>MAKKTLPAGVKSPPYIFSPIPFLGHAIAFGKSPIEFLENAYEKYGPVFSFTMVGKTFTYLLGSDAAALLFNSKNEDLNAEDVYSRLTTPVFGKGVAYDVPNPVFLEQKKMLKSGLNIAHFKQHVSIIEKETKEYFESWGESGEKNVFEALSELIILTASHCLHGKEIRSQLNEKVAQLYADLDGGFSHAAWLLPGWLPLPSFRRRDRAHREIKDIFYKAIQKRRQSQEKIDDILQTLLDATYKDGRPLTDDEVAGMLIGLLLAGQHTSSTTSAWMGFFLARDKTLQKKCYLEQKTVCGENLPPLTYDQLKDLNLLDRCIKETLRLRPPIMIMMRMARTPQTVAGYTIPPGHQVCVSPTVNQRLKDSWVERLDFNPDRYLQDNPASGEKFAYVPFGAGRHRCIGENFAYVQIKTIWSTMLRLY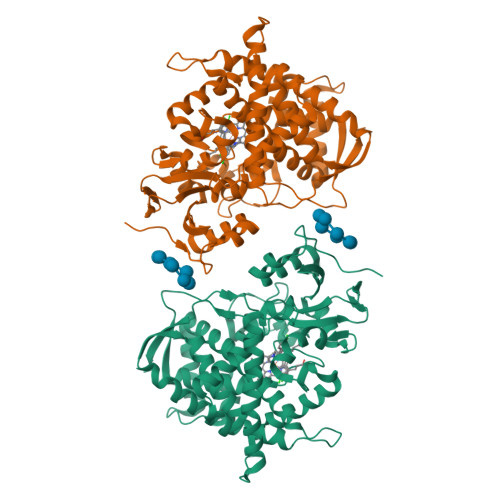EFDLIDGYFPTVNYTTMIHTPENPVIRYKRRSTHHHHHH[2x]>[4x]ASYGKKTQMSILEQRESLPIYKLKEQLVQAVHDNQILIVIGETGSGKTTQITQYLAEAGYTSRGKIGCTQPRRVAAMSVAKRVSEEFGCCLGQEVGYTIR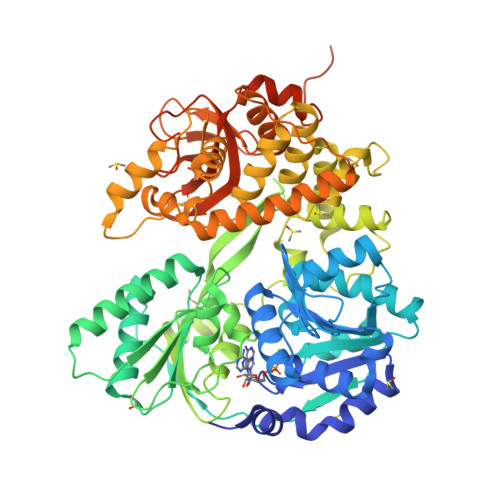FEDCTSPETVIKYMTDGMLLRECLIDPDLTQYAIIMLDEAHERTIHTDVLFGLLKKTVQKRQDMKLIVTSATLDAVKFSQYFYEAPIFTIPGRTYPVEILYTKEPETDYLDASLITVMQIHLTEPPGDILVFLTGQEEIDTACEILYERMKSLGPDVPELIILPVYSALPSEMQTRIFDPAPPGSRKVVIATNIAETSLTIDGIYYVVDPGFVKQKVYNSKTGIDQLVVTPISQAQAKQRAGRAGRTGPGKCYRLYTERAYRDEMLTTNVPEIQRTNLASTVLSLKAMGINDLLSFDFMDAPPMETLITAMEQLYTLGALDDEGLLTRLGRRMAEFPLEPMLCKMLIMSVHLGCSEEMLTIVSMLSVQNVFYRPKDKQALADQKKAKFHQTEGDHLTLLAVYNSWKNNKFSNPWCYENFIQARSLRRAQDIRKQMLGIMDRHKLDVVSCGKSTVRVQKAICSGFFRNAAKKDPQEGYRTLIDQQVVYIHPSSALFNRQPEWVVYHELVLTTKEYMREVTTIDPRWLVEFAPAFFKVSDPTKLSKQKKQQRLEPLYNRYEEPNAWRISRAFRRR>AQLCDQYATYTGGVYTINNNLWGKDAGSGSQCTTVNSASSAGTSWSTKWNWSGGENSVKSYANSGLTFNKKLVSQISQIPTTARWSYDNTGIRADVAYDLFTAADINHVTWSGDYELMIWLARYGGVQPIGSQIATATVDGQTWELWYGANGSQKTYSFVAPTPITSFQGDVNDFFKYLTQNHGF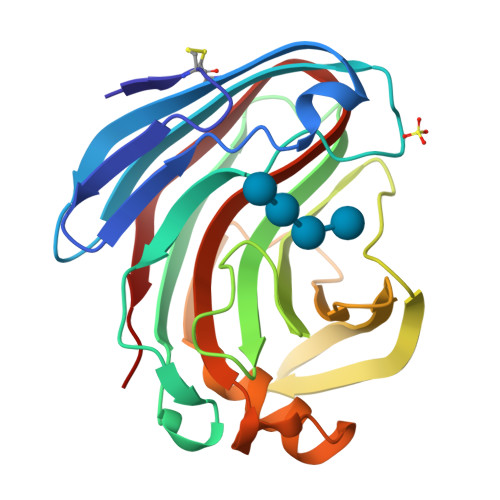PASSQYLITLQFGTAPFTGGPATLSVSNWSASVQ[7x]>MRSRRVDVMDVMNRLILAMDLMNRDDALRVTGEVREYIDT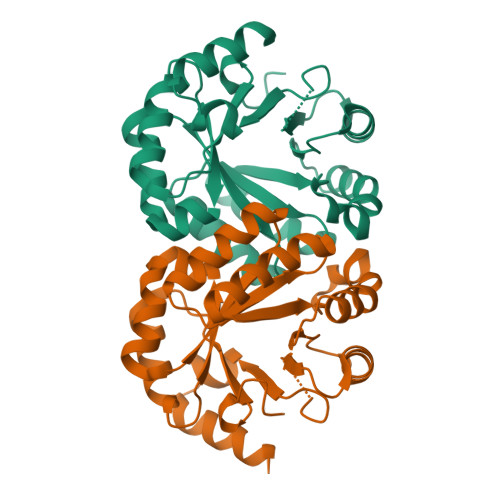VKIGYPLVLSEGMDIIAEFRKRFGCRIIADFKVADIPETNEKICRATFKAGADAIIVHGFPGADSVRACLNVAEEMGREVFLLTEMSHPGAEMFIQGAADEIARMGVDLGVKNYVGPSTRPERLSRLREIIGQDSFLISPGVGAQGGDPGETLRFADAAIVGRSIYLADNPAAAAAGIIESIKDLLNP[2x]> GMKITVVDLGNINVKYVGENKGRFSSKITNDYQSYEEGFQRVEYNGIKTYIGVGELSSREFNADRDYMAQLLYSLAKANTADTKEINLTLLLPIIQMKNKTRLIETLKGENFKFKFNGIDREIKINDLMVLPEGYASYYSLDDIENKGDVCILDLGSRTINICVLENAKIVKTNTIKLGSFDFYSKIKSLENAKGEDYIEEDIQDLIDNGLIKVDSKQYIEFLSDILNAVDPYVDLKTY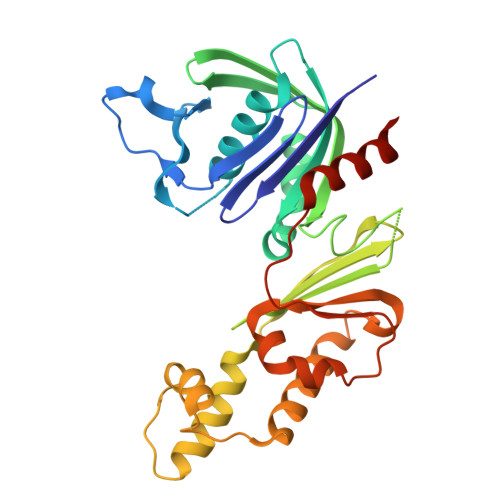NTIFTGGTSLMLKEYIEKLPLNKFKVHPNALTSNVDGAMEASKKVWNNNGN> MCYTGDPANNPLDRVRILCTDTNNDEILIEQSVLEWFYLESGKDEKKAAIKALKYLLFQVAKMGDEKVGGV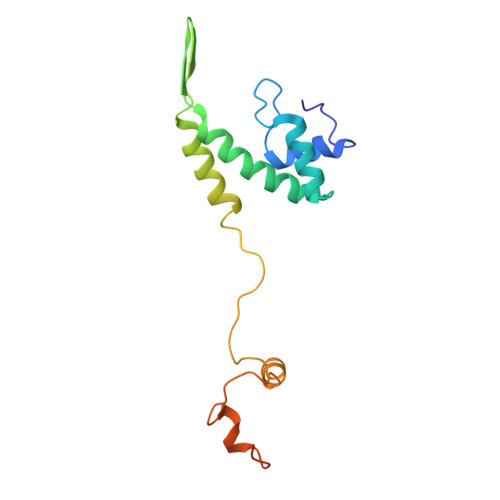YLRNSSRFKSLKAVYDDLVKSSVSGLPYAGGINQCDIDMRRQNPCSVKKYTEYGDAARYEGRDYCNRVNGVFIIERDE> KQTARKST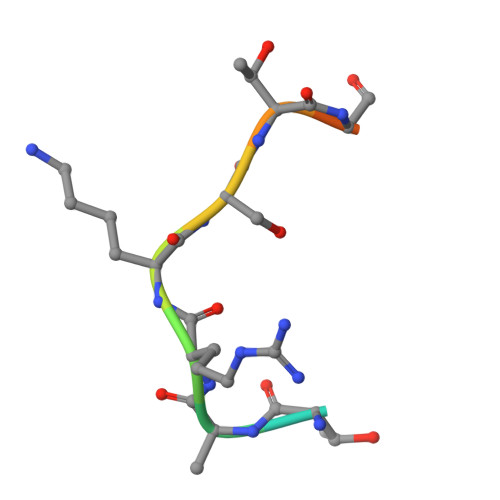GGKA N-Acetylpuromycin 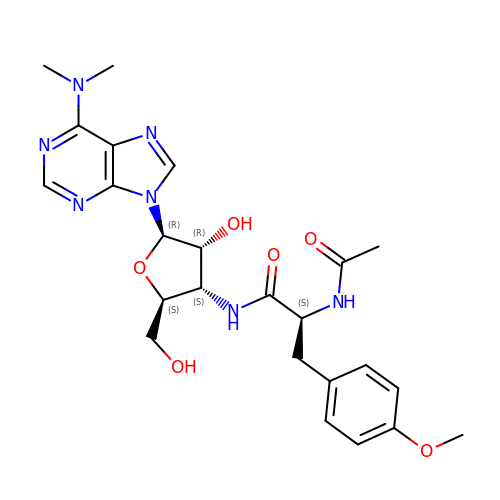| C24 H31 N7 O6 | LADKVYSQIGJMFP-IYRMOJGWSA-N>[2x]MSYDASAIRVLKGLEGVRHRPAMYIGGTGVEGYHHLFKEILDNAVDEALAGYATEILVRLNEDGSLTVEDNGRGIPVDLMPEEGKPAVEVIYNTLHSGGKFEQGAYKVSGGLHGVGASVVNALSEWTVVEVFREGKHHRIAFSRGEVTEPLRVVGEAPRGKTGTRVTFKPDPEIFGNLRFDPSKIRARLREVAYLVAGLKLVFQDRQHGKEEVFLDKGGVASFAK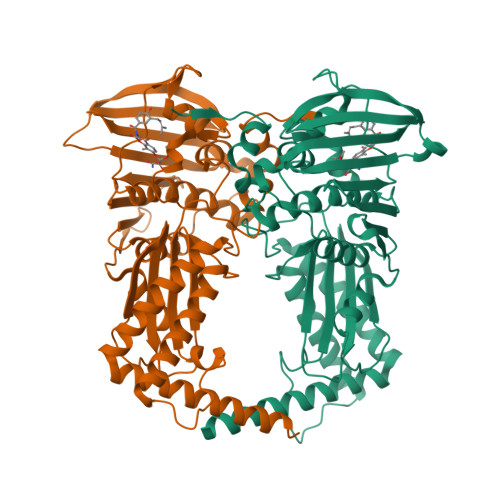ALAEGEDLLYEKPFLIRGTHGEVEVEVGFLHTQGYNAEILTYANMIPTRDGGTHLTAFKSAYSRALNQYAKKAGLNKEKGPQPTGDDLLEGLYAVVSVKLPNPQFEGQTKGKLLNPEAGTAVGQVVYERLLEILEENPRIAKAVYEKALRAAQAREAARKARELV>[2x]HHHHH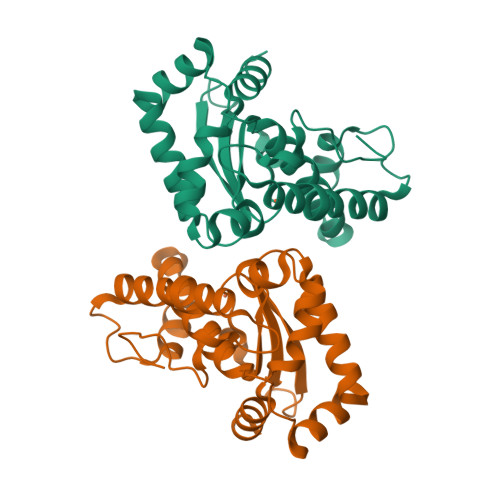HAPAELPKLGFNWKDGCAPVFSPRQMELHYTKHHKAYVDKLNALAGTTYDGKSIEEIILAVANDAEKKGLFNQAAQHFNHTFYFRCITPNGKAMPKSLESAVTAQFGSVEQFKDAFVQAGVNNFGSGWTWLCVDPSNKNQLVIDNTSNAGCPLTKGLRPVLAVDVWEHAYYKDFENRRPDYLKEIWSVIDWEFVAKMHAQAIK(2~{R},3~{R},4~{R})-2-(6-aminopurin-9-yl)-2-(hydroxymethyl)-5-methylidene-oxolane-3,4-diol 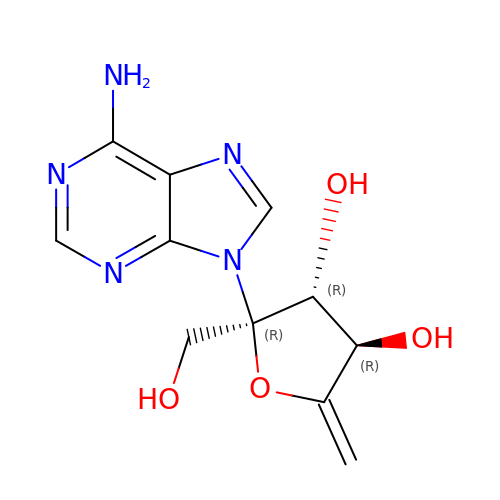| C11 H13 N5 O4 | UZSSGAOAYPICBZ-VAOFZXAKSA-N Schistosomiasis is the name of a severely debilitating disease caused by parasites of the genus Schistosoma, among which Schistosoma mansoni is the most prevalent species in the world and is estimated to infect approximately 200 million people. The parasite shows a complete dependence on preformed purines for its metabolic needs owing to an absence of the enzymes which comprise the ‘de novo’ pathway for purine biosynthesis. One key component of this pathway is the enzyme purine nucleoside phosphorylase (PNP), which catalyzes the reversible phosphorolysis of the N-ribosidic bond of 6-oxopurine deoxynucleosides and nucleosides yielding their correspondent base and ribose-1-phosphate. Crystal structures of several PNPs have been described which can be assigned to two main categories: the low-molecular-mass homotrimeric PNPs which bind to 6-oxopurines, and high-molecular-mass homohexameric PNPs that accept either 6-oxo or 6-aminopurine (such as adenosine) as substrates.

Aiming at shedding some further light on these questions we report for the first time the crystal structure of a binary complex between PNP and R1P alone. The asymmetric unit of the structure of SmPNP in complex with R1P (SmPNP–R1P) contains the full PNP trimer (6347 protein atoms) along with 368 water molecules, three molecules of R1P and three molecules of acetate. One possibility is the time used during the soaking experiment, which was much longer than that reported previously (48 h compared with a maximum of 2 h used for bovine PNP). The ligand presents an intricate hydrogen-bonding network involving either ten direct and four water-mediated hydrogen bonds (subunit A) or nine direct and five water-mediated hydrogen bonds (sub­units B and C). These interactions are limited to the well defined phosphate and ribose binding sites which are lined by residues S35, R86, H88, Y90, A118, Y202, M221, S222 and H259. The base binding site is occupied by one acetate molecule which interacts with E203 as described in previous SmPNP structures. c electron density map, as is frequently the case in other SmPNP structures. This suggests that the binding of R1P is not sufficient in itself to cause the loop rearrangement observed in complexes with the nucleosides inosine and adenosine. Even in subunits A and C, where the loop is well ordered, significant differences compared with the SmPNP–inosine structure can be seen. This is most notable for the interaction between O5′ of the ribose and H259 Nδ1, which is weaker in the SmPNP–R1P complex (3.4 Å and 3.07 Å in subunits A and C, respectively, compared with 2.73 Å and 2.62 Å in the SmPNP–inosine complex). The SmPNP–R1P complex is the first structure in which we observe a unique conformation for this loop suggesting that the anionic moiety may need to be covalently bound to the ribose in order to fully favour all interactions made by this loop.

>[3x]MHESVTANIENVKKVAHHIQKLTSIVPEIGIICGSGLGKLADGVKDKITIPYTKIPNFPQTSVVGHSGNLIFGTLSGRKVVVMQGRFHMYEGYSNDTVALPIRVMKLLGVKILMVSNAAGGLNRSLKLGDFVILKDHIYLPGLGLNNILVGPNQEAFGTRFPALSNAYDRDLRKLAVQVAEENGFGNLVHQGVYVMNGGPCYETPAECTMLLNMGCDVVGMSTIPEVVIARHCGIQVFAVSLVTNISVLDVESDLKPNHEEVLATGAQRAELMQSWFEKIIEKLPKD(3R)-1'-(9-ANTHRYLCARBONYL)-3-(MORPHOLIN-4-YLCARBONYL)-1,4'-BIPIPERIDINE | C30 H35 N3 O3 | 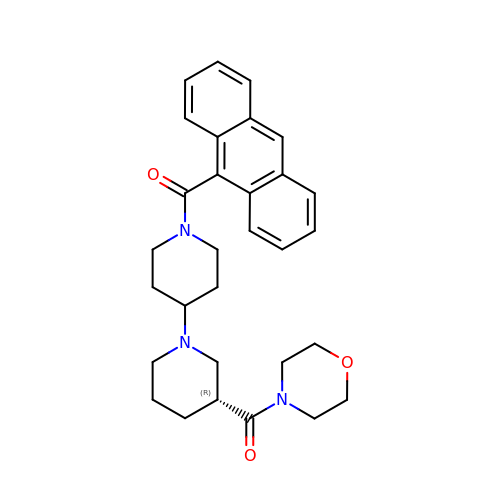LDQKDRLEMKIYMC-XMMPIXPASA-N>[5x]SLINTKIKPFKNQAFKNGEFIEVTEKDTEGRWSVFFFYPADFTFVCPTELGDVADHYEELQKLGVDVYSVSTDTHFTHKAWHSSSETIAKIKYAMIGDPTGALTRNFDNMRED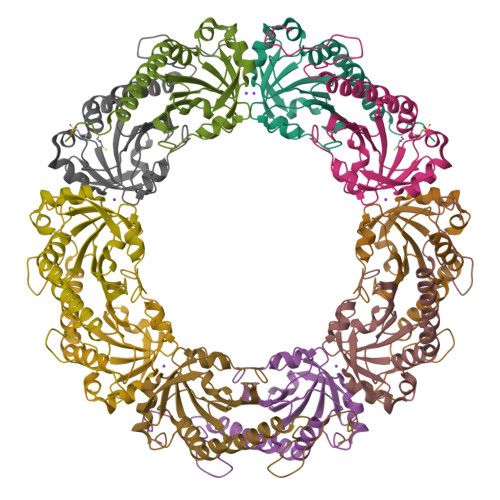EGLADRATFVVDPQGIIQAIEVTAEGIGRDASDLLRKIKAAQYVAAHPGEVSPAKWKEGEATLAPSLDLVGKI> MSKVFIATANAGKAHDADIFSVSACNSFTVSCSGDGYLKVWDNKLLDNENPKDKSYSHFVHKSGLHHVDVLQAIERDAFELCLVATTSFSGDLLFYRITREDETKKVIFEKLDLLDSDMKKHSFWALKWGASNDRLLSHRLVATDVKGTTY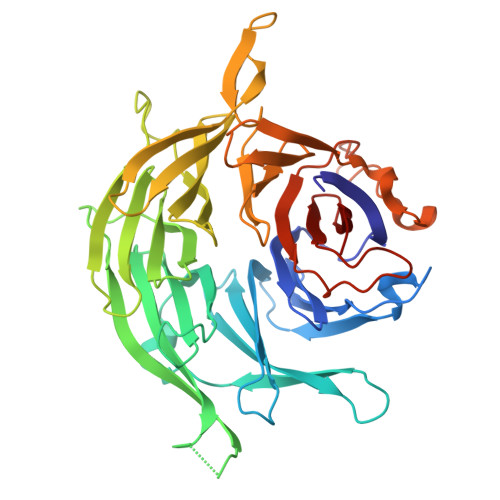IWKFHPFADESNSLTLNWSPTLELQGTVESPMTPSQFATSVDISERGLIATGFNNGTVQISELSTLRPLYNFESQHSMINNSNSIRSVKFSPQGSLLAIAHDSNSFGCITLYETEFGERIGSLSVPTHSSQASLGEFAHSSWVMSLSFNDSGETLCSAGWDGKLRFWDVKTKERITTLNMHCDDIEIEEDILAVDEHGDSLAEPGVFDVKFLKKGWRSGMGADLNESLCCVCLDRSIRWFREAGGK>GPGDPPATVYRYDSRPPEDVFQNGFTAWGNNDNVLEHLTGRSSQVGSSNSAFVSTSSSRRYTEVYLEHRMQEAVEAERAGRGTGHFIGYIY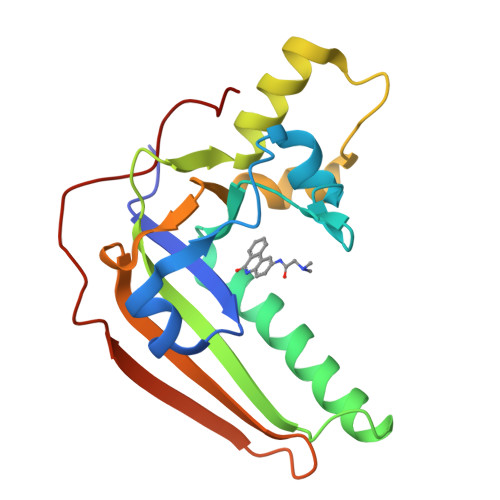EVRADNNFYGAASSYFEYVDTYGDNAGRILAGALATYQSEYLAHRRIPPENIRRVTRVYHNGITGETTTTEYSNARYVSQQTRANPNPYTS[2x]> MRKIVLPGDLLSTNPRAAGYGTYVEGGKVYAKIIGLFDQTETHVRVIPLKGRYTPSVGDVVIGIIREVAANGWAVDIYSPYQAFLPVSENPEMKPNKKPNEVLDIGDAIIAKVLNIDPKMKVTLTMKDRICRPIRFGRIVAINPARVPRVIGKKGSMIKLLKSELDVQIVVGQNGLIWVNGDRRKVSIAEEA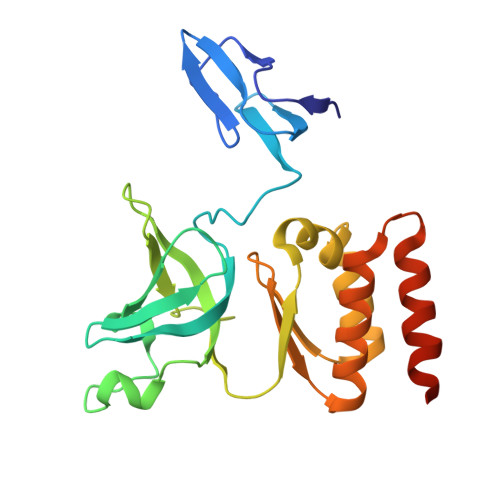IYLIEQEAHTEGLTDRVAEFIKRRKADVGIQHHHHHH>MNLQRFPRYPLTFGPTPIQPLARLSKHLGGKVHLYAKREDCNSGLAFGGNKTRKLEYLIPEALAQGCDTLVSIGGIQSNQTRQVAAVAAHLGMKCVLVQENWVNYSDAVYDRVGNIQMSRILGADVRLVPDGFDIGFRRSWEDALESVRAAGGKPYAIPAGCSDHPLGGLGFVGFAEEVRAQEAELGFKFDYVVVCSVTGSTQAGMVVGFAADGRADRVIGVDASAKPAQTREQITRIARQTAEKVGLERDIMRADVVLDERFAGPE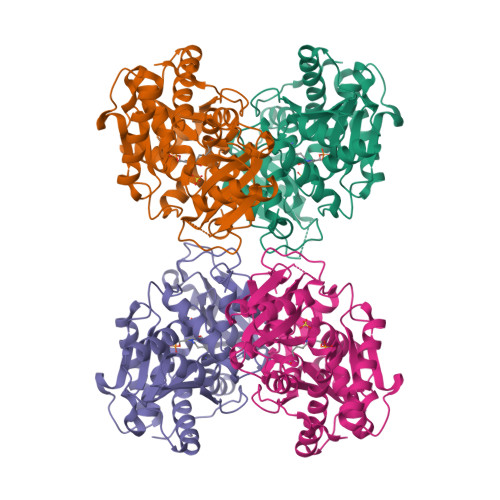YGLPNEGTLEAIRLCARTEGMLTDPVYEGKSMHGMIEMVRNGEFPEGSRVLYAHLGGVPALNGYSFIFRDG[4x]5'-O-{[2-(1H-indol-3-yl)ethyl]carbamoyl}guanosine 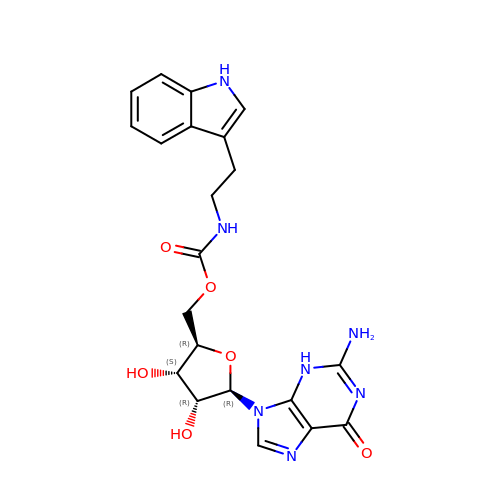| C21 H23 N7 O6 | WKHCFGWBMMFLHU-NVQRDWNXSA-N> MSCAGAAAAPRLWRLRPGARRSLSAYGRRTSVRFRSSGMTLDNISRAAVDRIIRVDHAGEYGANRIYAGQMAVLGRTSVGPVIQKMWDQEKDHLKKFNELMVTFRVRPTVLMPLWNVLGFALGAGTALLGKEGAMACTVAVEESIAHHYNNQIRTLMEEDPEKYEELLQLIKKFRDEELEHH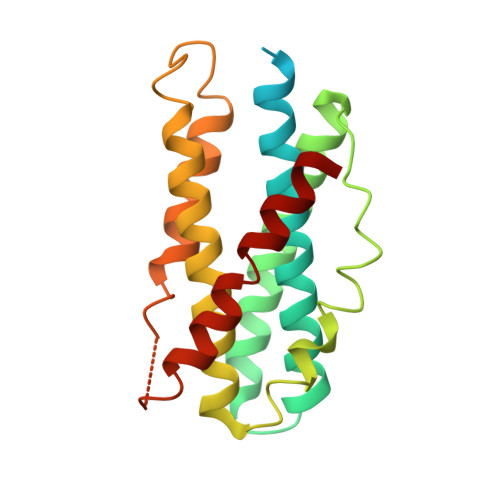DIGLDHDAELAPAYAVLKSIIQAGCRVAIYLSERL RNA ligases of the RTCB-type play an essential role in tRNA splicing, the unfolded protein response and RNA repair. RTCB is the catalytic subunit of the pentameric human tRNA ligase complex. RNA ligation by the tRNA ligase complex requires GTP-dependent activation of RTCB. This active site guanylylation reaction relies on the activation factor Archease.

To discern between the different conformations and oligomeric states, we crystallized human Archease (isoform 1; UniProtAC A8K0B5) and determined the X-ray structure at 1.84 Å resolution. The electrostatic surface potential of Archease is predominantly negative with a slightly positive region around the N-terminal helix. Residues 22–47 including helix 1 and β-strand 1 are located at positions equivalent to the swapped elements in the dimeric structure of human Archease. Helix 1 and the following loop possess high B-factors suggesting increased flexibility in this conserved region. No metal ion was bound in our Archease structure, unlike a previous structure of the PhArchease dimer, which harbors a calcium ion. Formation of the RTCB-Archease complex, as presented here, is only possible with the monomeric form of Archease due to the sterical clash with a strand-swapped dimer. While our results do not exclude a functional role of dimerization in vivo, they support the monomeric form of Archease as the functionally active state.

> GSHMMKGGSRVSNPAVMAQEEEDVRDYNLTEEQKAIKAKYPPVNRKYEYLDHTADVQLHAWGDTLEEAFEQCAMAMFGYMTDTGTVEPLQTVEVETQGDDLQSLLFHFLDEWLYKFSADEFFIPREVKVLSIDQRNFKLRSIGWGEEFSLSKHPQGTEVKAITYSAMQVYNEENPEVFVIIDI muvalaplin  | C42 H54 N4 O6 | 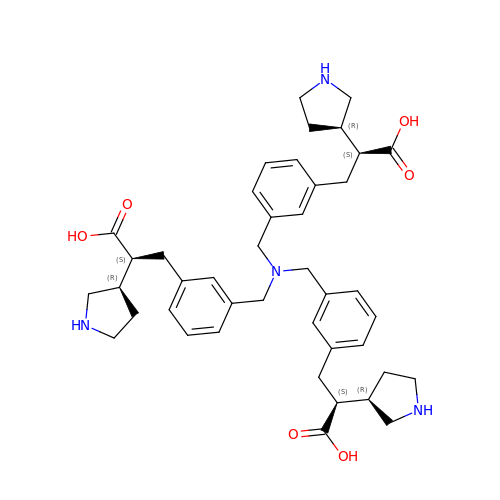BRLGERLDHZRETI-BGBFCPIGSA-N> SANEDMPVERILEAELAVEPKTETYVEANMGLNPSSPN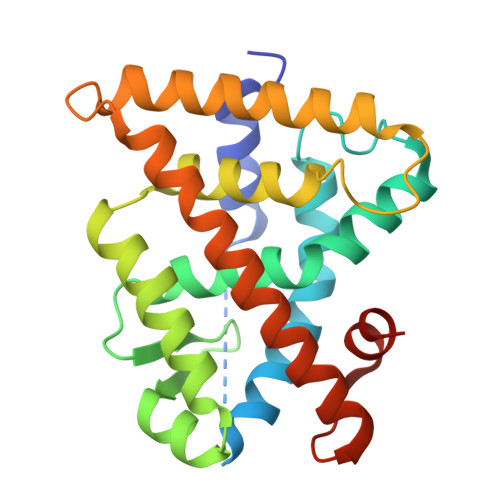DPVTNICQAADKQLFTLVEWAKRIPHFSELPLDDQVILLRAGWNELLIASFSHRSIAVKDGILLATGLHVHRNSAHSAGVGAIFDRVLTELVSKMRDMQMDKTELGCLRAIVLFNPDSKGLSNPAEVEALREKVYASLEAYCKHKYPEQPGRFAKLLLRLPALRSIGLKCLEHLFFFKLIGDTPIDTFLMEMLEAPHQMT PANTOYL ADENYLATE | C16 H24 N5 O10 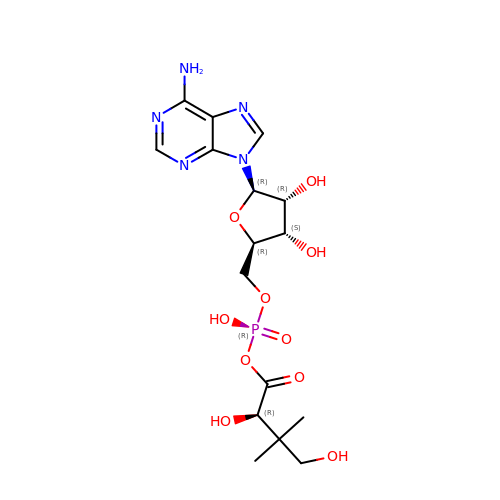P | GDPVENOGSVMRJL-FSRKKXLISA-N> DDFRVGERVWVNGNKPGFIQFLGETQFAPGQWAGIVLD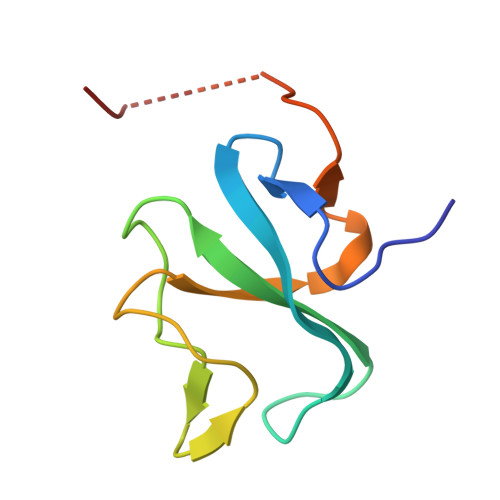EPIGKNDGSVAGVRYFQCEPLKGIFTRPSKLTRKVQAEDEANGLQTTP In this study, the effect of physical and chemical factors on the orientations of macromolecules was investigated through an analysis of selected well studied macromolecules, and important parameters that determine the behaviour of proteins on cryo-EM grids were revealed. The test proteins used in the analysis include human C-reactive protein (CRP) pentamer, CRP decamer, human erythrocyte catalase, SARS-CoV-2 spike protein, E. coli PaaZ and E. coli β-galactosidase. We performed a comprehensive examination of how macromolecule orientations respond to alterations in physical factors, such as freezing temperature, and chemical factors, such as the addition of surfactants or the presence of affinity tags, during grid freezing for a standard set of proteins. Hence, electrostatic interactions at the AWI are an important factor in determining protein orientations in the absence of any additive.

CRP exists in a concentration-dependent equilibrium between a pentamer and a decamer of a 25 kDa polypeptide under physiological conditions. In the concentration range used for cryo-EM experiments, both pentamer and decamer populations were observed in the same micrograph and were analysed separately. C5 symmetry was applied to the smaller pentameric molecule and no symmetry was applied to the decamer during image processing. The CRP decamer and SARS-CoV-2 spike had a more severe orientation bias, with more than 90% abundance of the preferred view, whereas in the case of the CRP pentamer the abundance was 50% and in catalase it was near 60%. The negatively charged B-face of CRP in the absence of additive is less sampled in the case of the CRP pentamer and is not sampled at all in the CRP decamer. However, this scenario does not seem to be applicable to CRP, as both the pentamer and decamer populations adopt preferred orientations in the absence of additives, indicating their interaction with the AWI. The orientations observed in this case look similar and the resulting reconstructions from 256 289 and 204 354 particles for the pentamer and decamer (C5 and C1 symmetry) resulted in resolutions of 3.2 and 2.8 Å, respectively. In comparison, we have obtained a 3.3 Å resolution map for the pentamer and a 4 Å resolution map for the decamer by averaging 25 000 and 51 000 particles, respectively.

>[10x]MEKLLCFLVLTSLSHAFGQTDMSRKAFVFPKESDTSYVSLKAPLTKPLKAFTVCLHFYTELSSTRGYSIFSYATKRQDNEILIFWSKDIGYSFTVGGSEILFEVPEVTVAPVHICTSWESASGIVEFWVDGKPRVRKSLKKGYTVGAEASIILGQEQDSFGGNFEGSQSLVGDIGNVNMWDFVLSPDEINTIYLGGPFSPNVLNWRALKYEVQGEVFTKPQLWP Here we report the synchronous behavior of the adenine riboswitch aptamer RNA in crystal during ligand-triggered isothermal phase transitions. Here we report the interplay of synchronous molecular conformational changes and ordered SS transitions in crystals of adenine riboswitch aptamer RNA (riboA), elucidated using a multidisciplinary approach. Using a combination of methods—PVM, AFM, and XFEL—the results of this study demonstrate, in real time, the synchrony of molecular changes that occur in the ligand-induced phase transition of riboA crystals.

Unit-cell measurements identified three primary lattices, defined as apo unit cell (AUC), transition unit cell 1 (TUC1), and bound unit cell (BUC). The first transition, AUC to TUC1, is measurable by the change in the c-axis from 9.3 to 7.9 nm. With increasing delay time, the indexing rate for AUC falls off steeply with a coincident emergence of the pseudo-monoclinic transitional unit cell, TUC1. Importantly, Bragg diffraction is maintained throughout the entire transition from AUC to TUC1, with very little change in the diffraction hit-rate, and no evidence of crystals becoming completely disordered or entering the liquid phase. At 10 s, an additional set of Bragg peaks emerges corresponding to a (50.3 Å) and b (25.2 Å) dimensions of TUC1, which become more prominent with increasing delay time. The presence of peaks corresponding to TUC1 in the 3D reciprocal lattices merged with respect to AUC-indexed orientations indicates that the TUC1 diffraction comes from AUC-indexed and oriented crystals. Upon manual inspection of individual diffraction patterns, numerous images exhibited such differentiated AUC and TUC1 lattices in the same crystals, illustrating the sudden yet cooperative behavior of T1, corroborating the PVM and AFM results. In the a*c* plane, the rapid sampling by TRX reveals azimuthal streaks about b* at 10 s, whose degree of elongation increases at 25 s, and coincides with the shortening of the c-axis (from 93.4 to 78.7 Å) and the change in the unique angle of the monoclinic cell (from β to α). Based on the sequential appearance in both PVM and AFM, T1 observed by PVM corresponds to the AUC–TUC1 lattice transition, whereas T2 and T3 are likely related to the transitions from TUC1 to TUC2, and from (TUC1/TUC2) to BUC.

>[2x]GGGAAGAUAUAAUCCUAAUGAUAUGGUUUGGGAGUUUCUACCAAGAGCCUUAAACUCUUGAUUAUCUUCCC>SNAAGFAQASPSAPVAGKDFEVMKSPQPVSAPAGKVEVIEFFWYGCPHCYEFEPTIEAWVKKQGDKIAFKRVPVAFRDDFVPHSKLFYALAALGVSEKVTPAVFNAIHKEKNYLLTPQAQADFLATQGVDKKKFLDAYNS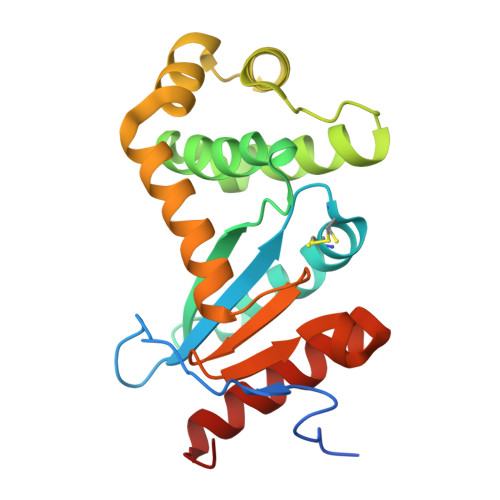FSVQGQVKQSAELLKNYNIDGVPTIVVQGKYKTGPAYTNSLEGTAQVLDFLVKQVQDKKL[4x]>[4x]MDSLDQCIVNACKNS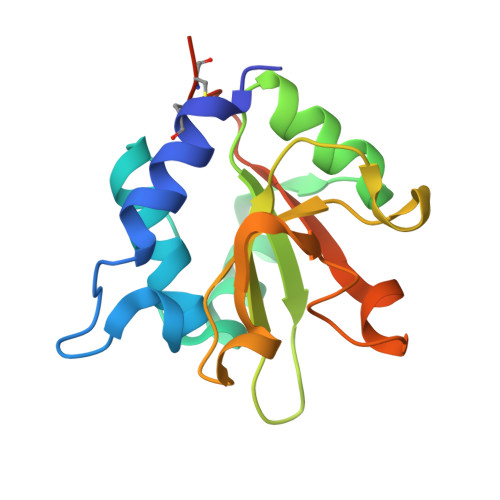WDKSYLAGTPNKDNASGFVQSVAAELGVPMPRGNANAMVDGLEQSWTKLASGAEAAQKAAQGFLVIAGLKGRTYGHVAVVISGPLYRQKYPMCWCGSIAGAVGQSQGLKSVGQVWNRTDRDRLNYYVYSLASCSLPRASHHHHHH> MEKTRVNGTDRPPISSWSVDDVSNFIRELPGCQDYVDDFIQQEIDGQALLLLKEKHLVNAMGMKLGPARKIVAKVESIKEVRDHHH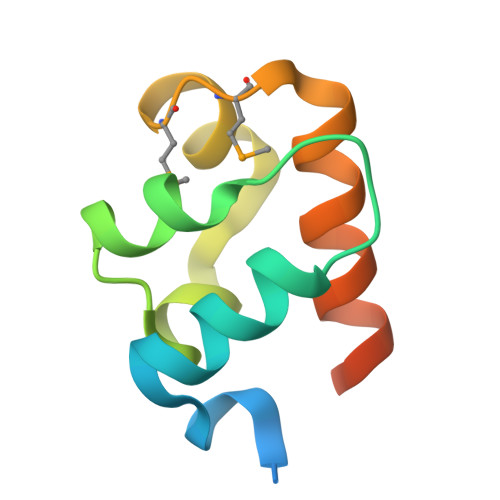HHH> CG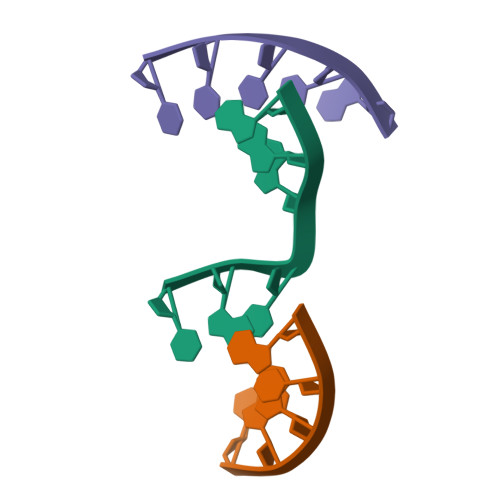ACG;> TCCTA;> CGTGGA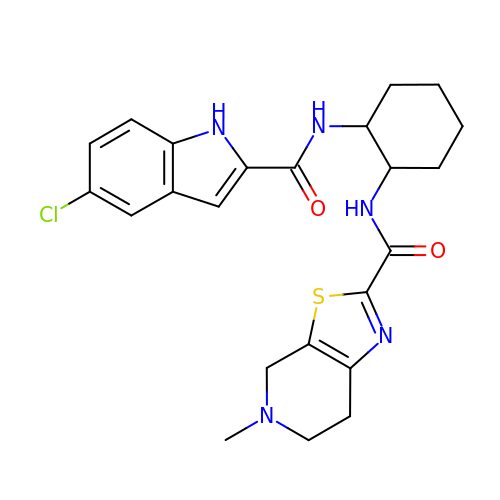N-((1R,2S)-2-(5-CHLORO-1H-INDOLE-2-CARBOXAMIDO)CYCLOHEXYL)-5-METHYL-4,5,6,7-TETRAHYDROTHIAZOLO[5,4-C]PYRIDINE-2-CARBOXAMIDE | C23 H26 Cl N5 O2 S | ARPFWVKYXJZULB-DLBZAZTESA-N> ANSANTNTVPKLYRSV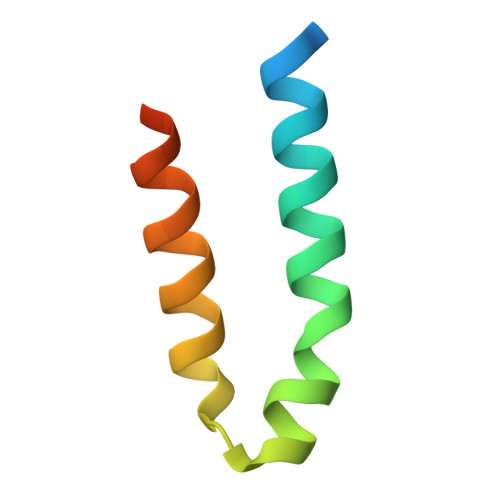IEDVINDVRDIFLDDGVDEQVLMELKTLWENKLMQSRAVDG>[2x]MKVSLMAAKAKNGVIGCGPHIPWSAKGEQLLFKALTYNQWL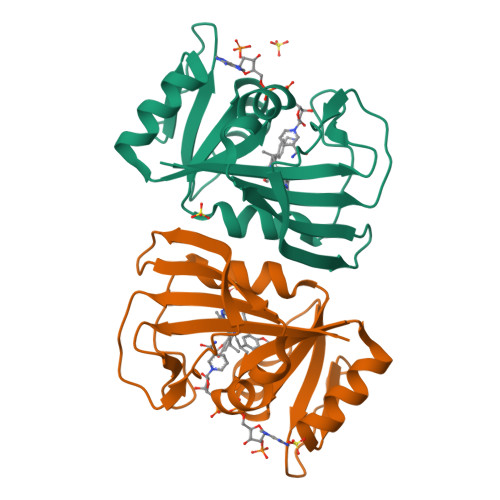LVGRKTFESMGALPNRKYAVVTRSAWTADNDNVIVFPSIEEAMYGLAELTDHVIVSGGGEIYRETLPMASTLHISTIDIEPEGDVFFPNIPNTFEVVFEQHFSSNINYCYQIWQKG EDA is a tumor necrosis factor (TNF) family member, which functions together with its cognate receptor EDAR during ectodermal organ development. Mutations of EDA have long been known to cause X‐linked hypohidrotic dysplasia in humans characterized by primary defects in teeth, hair and sweat glands. EDA·A1 and EDA·A2 interact with two distinct receptors EDAR and XEDAR respectively via binding of their THDs to the cysteine-rich domains (CRDS) in their receptors. Here, we report the crystal structure of EDA C-terminal TNF homology domain bound to the N-terminal cysteine-rich domains of EDAR.

To reveal the structural basis for the interaction between EDA·A1THD and EDARCRDS, we crystallized the EDA·A1THD-EDARCRDS complex and determined its structure using the single-wavelength anomalous dispersion (SAD) method at a resolution of 2.8 Å. The crystal structure reveals that EDA·A1THD and EDARCRDS form a heterohexameric complex, displaying a triangular-shaped architecture with an EDA·A1THD trimer in the center and three EDARCRDS molecules at the vertexes of the complex. The structure of the THD trimer in the complex is almost identical to that of the crystal structure of the apo EDA·A1, indicating that binding to the receptor does not cause substantial structural changes of the ligand. Each EDARCRDS molecular binds across the convex surface of a single EDA·A1THD in the trimer, burying about 1340 Å2 of total solvent accessible surface area at the intermolecular interface. The 1:1 binding mode between EDA·A1 and EDAR is markedly different from those previously observed in other TNF-receptor complex structures, such as TNF-TNFR2 and RANKL-RANK, in which each receptor binds into the concaved groove formed by two adjacent ligand protomers of the receptor. At the EDA·A1THD-EDARCRDS interface, although all three CRDs of EDAR form direct contacts with EDA·A1THD, the second CRD mediates most of the interactions with the ligand. The driving force for the binding of EDA·A1THD to EDARCRDS is predominantly electrostatic interactions via three pairs of charged patches on the surfaces of the receptor and the ligand with complementary electrostatic potentials. A cluster of acidic and polar residues in EDA·A1THD (Gln256, Gln261, Asp265, Asp273) mediate a panel of electrostatic interactions with positively charged residues in EDARCRD2 (Lys78, Arg88, Arg89), tightly tethering antiparallel β3-β4 motif of EDARCRDS to the surface of EDA·A1THD. Instead, the presence of Val307 and Glu308 extend the length of strand βC of EDA·A1THD so that the aromatic sidechains of Tyr310, Try311 and Tyr343 pack together to form a hydrophobic patch that makes intimate contacts with helix α1 from EDARCDR2. Our crystal structure predicts that a glutamate substitution of Ala259 would severely deform the saddle-shaped depression of EDA·A1 whereas a glycine replacement of Asp265 reduces the acidic surface area at the interface.

>[2x]GPSGAADKAGTRENQPAVVHLQGQGSAIQVKNDLSGGVLNDWSRITMNPKVFKLHPRSGELEVLVDGTYFIYSQVEVYYINFTDFASYEVVVDEKPFLQCTRSIETGKTNYNTCYTAGVCLLKARQKIAVKMVHADISINMSKHTTFFGAIRLGEAPAS;> YSNCGENEYYNQTTGLCQECPPCGPGEEPYLSCGYGTKDEDYGCVPCPAEKFSKGGYQICRRHKDCEGFFRATVLTPGDMENDAECGPCLPGYYMLENRPRNIYGMVCYSCLLAPPNTKECVG>KKEDVTLVLTEENFDEVIRNNKLVLVDCWAEWCAPCHLYEPIYKKVAEKYKGKAVFGRLNVDEN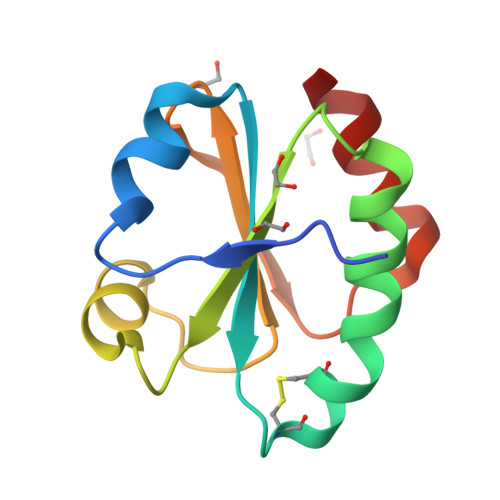QKIADKYSVLNIPTTLIFVNGQLVDSLVGAVDEDTLESTVNKYLK[3x]>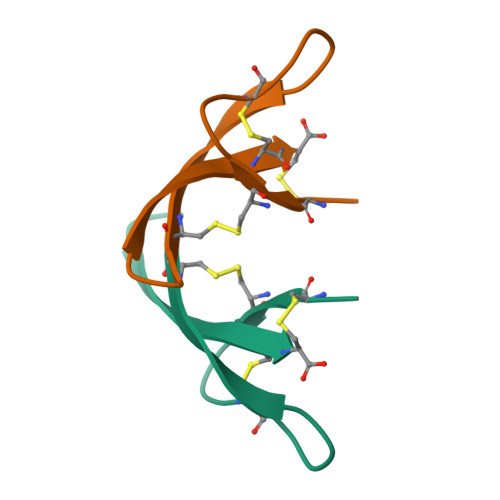DCYCRIPACIAGEKKYGTCIYQGKLWAFCC[2x]> AIVNSVDTMTLTNANVSPDGFTRAGILVNGVHGPLIRGGKNDNFELNVV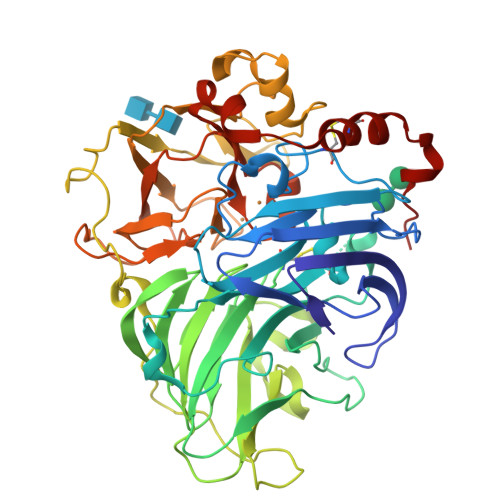NDLDNPTMLRPTSIHWHGLFQRGTNWADGADGVNQCPISPGHAFLYKFTPAGHAGTFWYHSHFGTQYCDGLRGPMVIYDDNDPHAALYDEDDENTIITLADWYHIPAPSIQGAAQPDATLINGKGRYVGGPAAELSIVNVEQGKKYRMRLISLSCDPNWQFSIDGHELTIIEVDGELTEPHTVDRLQIFTGQRYSFVLDANQPVDNYWIRAQPNKGRNGLAGTFANGVNSAILRYAGAANADPTTSANPNPAQLNEADLHALIDPAAPGIPTPGAADVNLRFQLGFSGGRFTINGTAYESPSVPTLLQIMSGAQSANDLLPAGSVYELPRNQVVELVVPAGVLGGPHPFHLHGHAFSVVRSAGSSTYNFVNPVKRDVVSLGVTGDEVTIRFVTDNPGPWFFHCHIEFHLMNGLAIVFAEDMANTVDANNPPVEWAQLCEIYDDLPPEATSIQTV> NITIYHNPACGTSRNTLEMIRNSGTEPTIILYLENPPSRDELVKLIADMGISVRALLAKNVEPYEQLGLAEDKFTDDQLIDFMLQHPILINRPIVVTPLGTRLCRPSEVVLDI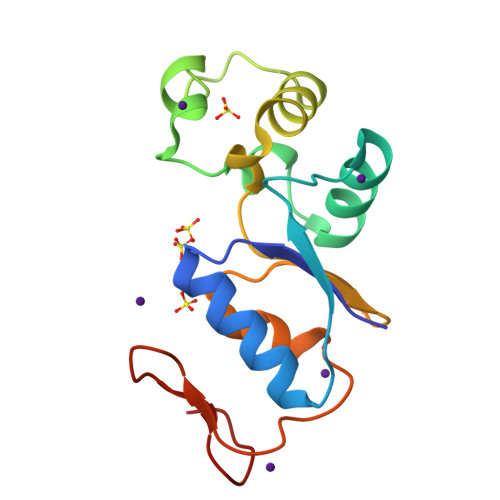LQDAQKGAFTKEDGEKVVDEAGKRL> MTNTLQVKLLSKNARMPERNHKTDAGYDIFSAETVVLEPQEKAVIKTDVAVSIPEGYVGLLTSRSGVSSKTHLVIETGKIDAGYHGNLGINIKNDHEDDKMQTIFLRNIDNEKIFEKERHLYKLGSYRIEKGERIAQLVIVPIWTPELKQVEEFESVSERGEKGFGSSGV

We have recently proposed that the trimeric staphylococcal phage encoded dUTPases (Duts) are signaling molecules that act analogously to eukaryotic G-proteins, using dUTP as a second messenger. To initiate the SaPI cycle, a specific phage-encoded protein binds to the SaPI-encoded repressor Stl, acting as an antirepressor. Both the trimeric and the dimeric phage-encoded Dut proteins are the antirepressor proteins for a subset of SaPIs, including SaPIbov1, SaPIbov5 or SaPIov1 (8–10). However, our results analyzing the Dut protein from phage 80α (Dut80α) revealed that motif VI is essential for interaction with the SaPI-encoded Stl repressor, determining the affinity with which the Dut proteins bind to the Stl repressor.

We thought that the differential effect of each nucleotide could be related to the mechanism of Stl binding and we tried to clarify this ambiguity using two complementary strategies: first, we solved the structure of the Dut80α bound to dUMP; next, we analyzed the formation of the Stl:Dut complex in the presence of dUMP. Remarkably, the structure of the Dut80αWT bound to the dUMP showed that motif V was ordered over the active site. Comparison with the structure of Dut80α bound to dUPNPP shows a slight but evident difference in the conformation of motif V, that affects the last four C-terminal residues. This partially conserved region (GSSGV) of the C-terminal motif V, which is involved in γP recognition and enzyme activity, adopts an alternative conformation in the presence of dUMP, approaching motif VI. The reported fast posthydrolysis release of dUTP products, pyrophosphate and dUMP, in Duts would also be favored by the weaker dUMP stabilization of motif V over the active center as is reflected by the B-factors increment of this region (30% higher for motif V than for Dut main body) and the absence of density for the final two residues on dUMP-bound Dut80α. Interestingly, the dUMP-induced motif V conformation was similar to one of our previously characterized Dut80α mutants, in this case the Dut80α D81A D110C S168C (in short Dut80αD81A C-C). And in agreement with the results obtained by Szabo et al. with Dutϕ11 (13), the dUMP does not interfere with the formation of the Stl:Dut80α complex. In summary, while the crystallographic data show that dUMP induces conformational changes in the C-terminal part of motif V, the affinity of the Dut:Stl complex is not increased in the presence of this nucleotide, suggesting that this change neither favors nor hampers the interaction with the repressor. Indeed, the analyzed motif IV residues are in close vicinity of the pyrophosphate and C- terminal part of motif V, the two elements that show changes (the first is absent and the second alter its conformation), depending on whether it is the dUMP or the dUTP that is bound to the enzyme.>MENSDDIRLIVKIAQLYYEQDMTQAQIARELGIYRTTISRLLKRGREQGIVTIA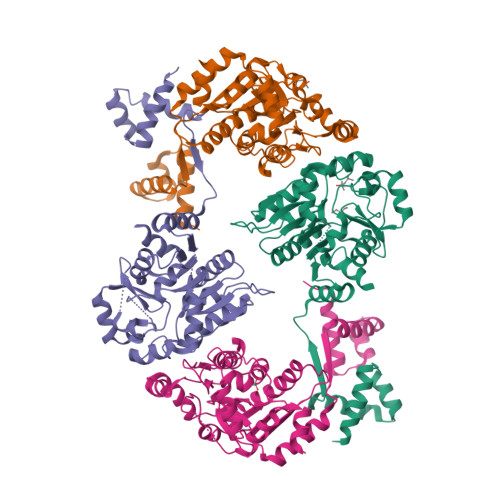INYDYNENLWLEQQLKQKFGLKEAVVASSDGLLEEEQLSAMGQHGALLVDRLLEPGDIIGFSWGRAVRSLVENLPQRSQSRQVICVPIIGGPSGKLESRYHVNTLTYGAAARLKAESHLADFPALLDNPLIRNGIMQSQHFKTISSYWDSLDVALVGIGSPAIRDGANWHAFYGSEESDDLNARHVAGDICSRFYDINGGLVDTNMSEKTLSIEMAKLRQARYSIGIAMGEEKYSGILGALHGRYINCLVTNRETAELLLK[4x]> 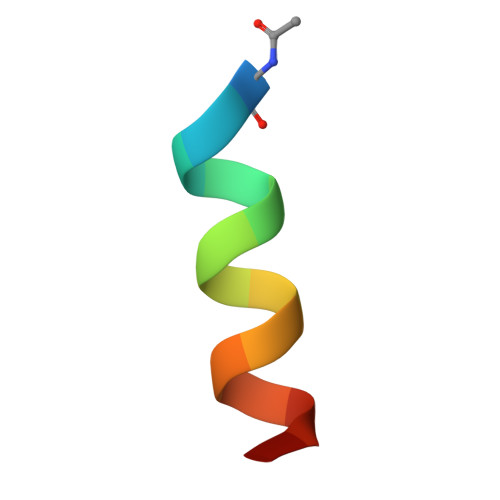XAIAEQLRAIGDAFX> GPLGSPEFMALAVAPWGRQWEEARALGRAVRMLQRLEEQCVDPRLSVSPPSLRDLLPRTAQLLREVAHSRRAAGGGGPGGPGGSGDFLLIYLANLEAKSRQVAALLPPRGRRSANDELFRAGSRLRRQLAKLAIIFSHMHAELHALFPGGKYCGHMYQLTKAPAHTFWRESCGARCVLPWAEFESLLGTCHPVEPGCTALALRTTIDLTCSGHVSIFEFDVFTRLFQPWPTLLKNWQLLAVNHPGYMAFLTYDEVQERLQACRDKPGSYIFRLSCTRLGQWAIGYVSSDGSILQTIPANKPLSQV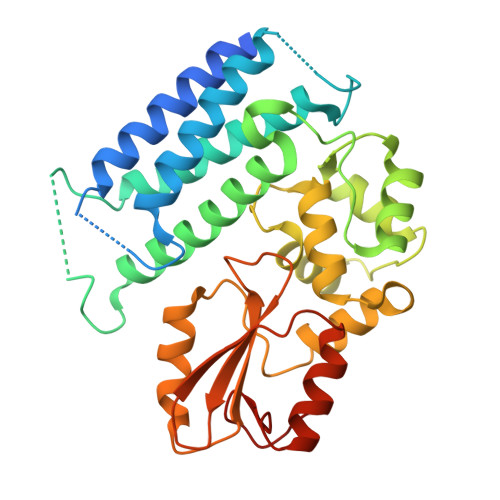LLEGQKDGFYLYPDGKTHNPDLTELG4-azanyl-6-[[(1~{S})-1-[6-[3-[(dimethylamino)methyl]phenyl]-3-methyl-5-oxidanylidene-[1,3]thiazolo[3,2-a]pyridin-7-yl]ethyl]amino]pyrimidine-5-carbonitrile 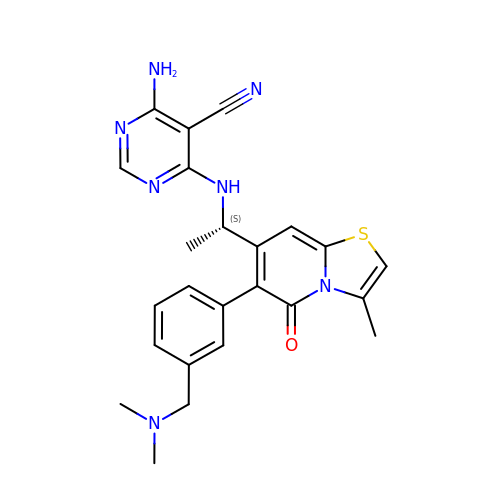| C24 H25 N7 O S | OQIHNLNLZCEEGI-HNNXBMFYSA-N> MGSDKIHHHHHHMNTPREVTLHFLRTAGHPL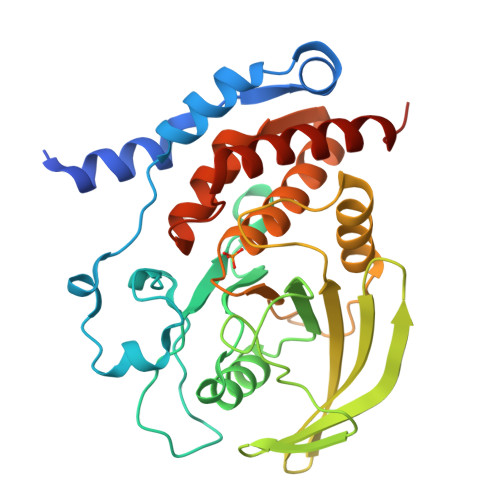TRWALQRQPPSPKQLEEEFLKIPSNFVSPEDLDIPGHASKDRYKTILPNPQSRVCLGRAQSQEDGDYINANYIRGYDGKEKVYIATQGPMPNTVSDFWEMVWQEEVSLIVMLTQLREGKEKCVHYWPTEEETYGPFQIRIQDMKECPEYTVRQLTIQYQEERRSVKHILFSAWPDHQTPESAGPLLRLVAEVEESPETAAHPGPIVVHSSAGIGRTGCFIATRIGCQQLKARGEVDILGIVCQLRLDRGGMIQTAEQYQFLHHTLALYAGQLPEEPSP>[6x]MNDSRNSGTLAVLVHGAWHSSLHWAAAQRGLARRGVASIAVDLPGHGLDAPVPSGYLTAGQPGLETEKSALADITMDDLADAVVDALAEVRSRFARVLLVAHSAGGGPASLAAEKAPELVDHLVYLAAFVPAARPRFTDYINAPENADVVALPIFSDPANLGAHRLNPLSSDAIEVDAIRRAFLTDMPPDAPEGWRHLLHPDEPYASLSAPVPVTPRRWGRIPRTYIRLDGDRALAPTTQNLM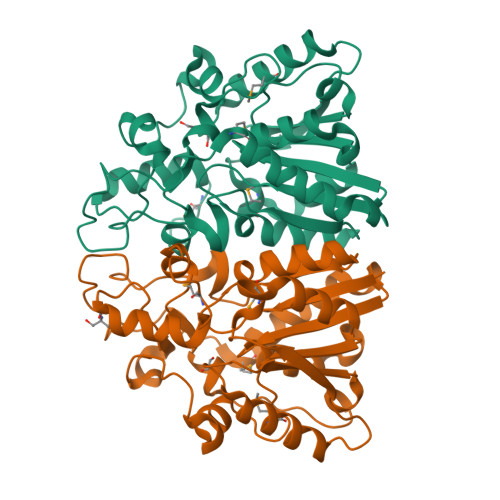IAEADRLTPDNPFGVRSLPGDHSPMVHRPGELADLLAGI>MHHHHHHAGNSILLAAVSILSACQQSYFALQVGKARLKYKVTPPAVTGSPEFERVFRAQQNCVEFYPIFIITLWMAGWYFNQVFATCLGLVYIYGRHLYFWGYSEAAKKRITGFRLSLGILALLTLLGALGIANSFLDEYLDLNIAKKLRRQF[6x]

Microsomal glutathione S-transferase 2 (MGST2) is a member of a family of integral membrane proteins denoted MAPEG (Membrane Associated Proteins in Eicosanoid and Glutathione metabolism), which encompasses several important targets for development of anti-inflammatory and anti-cancer drugs interfering with prostaglandin and leukotriene biosynthesis. In non-hematopoietic cells, MGST2 catalyzes leukotriene C4 (LTC4) synthesis via conjugation of glutathione (GSH) and LTA4, a transient epoxide intermediate derived from 5-lipoxygenase metabolism of arachidonic acid. Previous studies of MGST2 have revealed that only one out of three active sites is used at a time, an intriguing catalytic behavior also observed for MGST1 and microsomal prostaglandin E synthase-1 (mPGES-1) both of which are strongly implicated in human pathophysiology. The overall structure is a homo-trimer, with each monomer containing 4 trans-membrane α-helices (αH1–αH4), forming three potential active sites at their interfaces.

The structure of apo-MGST2 (with two homo-trimers in the asymmetric unit) shows structural heterogeneity, while the structure of holo-MGST2, which contains GSH at only two of the three possible active sites appears more rigid. Specifically, the four-residue stretch (Ala101–Arg104) at the beginning of αH4, which forms part of the active site and contains the catalytically important Arg104, is uniformly observed in a 310 helical motif within the apo structure and the GSO3− complex. Notably, Asn55 on αH2 forms an intra-monomeric interaction with Arg90 on αH3 in the apo structure while it moves toward GSH in the holo structure. However, we observed significant structural differences in pore-lining residues between the apo and holo states: for instance, reorientation in the side chain of Val57 upon GSH binding broadens the cytoplasmic side of the cavity possibly increasing solvent access. In apo simulations on a membrane, the symmetry of inter-subunit interactions early breaks and the 310 helix at the active site unfolds in one unit at a time. Moreover, such unfolding is also reversible with some runs undergoing transient refolding. This local unfolding is not subunit-specific, occurring in a different monomer in each replica trajectory, and is accompanied by changes in inter-subunit contacts. In the apo state, 310 helix unfolding coupled with αH4 tilting is accompanied by further structural changes: loop L opens, Pro61 kink unfolds, the kink angle increases, and Trp-gate opens. These conformational changes widen the central pore, allow a significant water influx throughout the inner cavity, and expose the active site to solvent. In this state, the highly dynamic loop L, which protrudes to the solvent, can trap GSH and help approximate it to the binding site.The recombinant MacQ protein exhibited bifunctional acylase activity against various ranges of AHLs and against multiple β-lactam antibiotics, including penicillin G, ampicillin, and amoxicillin. The MacQ protein is comprised of 806 amino acid residues, including an N-terminal signal peptide, and belongs to the N-terminal nucleophile (Ntn) hydrolase superfamily. AHL-acylase is one of the enzymes capable of inactivating AHLs via hydrolysis of the amide bond of the acyl side-chain to produce homoserine lactone (HSL) and fatty acid. The MacQ structure clearly revealed a typical Ntn-hydrolase fold comprised of a four-layered α-β-β-α motif45 mainly composed of two polypeptide chains, α- and β-chains, generated by self-cleaving activity.

The crystal structures of MacQ, both ligand-free and in complex with the reaction products of decanoic acid (C10) and phenyl acetic acid (PAA), were determined at 2.6 Å, 2.2 Å, and 1.75 Å resolution, respectively. First, electron density was observed for the SP lying in the vicinity of the active-site pocket. This was quite unexpected, because the SP was not found in any previously reported structures of penicillin G/cephalosporin/AHL-acylases and is believed to fall away in the course of the autoproteolytic maturation. The SP atoms were refined with full occupancy, while the B-factor values of the SP were relatively high compared to those of α- and β-chain, indicating increased conformational heterogeneity or a lower occupancy of the SP as compared to the α- and β-chains. Second, the crystal structure analysis revealed that MacQ forms a high oligomeric quaternary structure. The two heterodimers consisting of the α- and β-chain are arranged face-to-face, resulting in the formation of an approximately 170-kDa capsule-shaped molecule (dimer of heterodimer) containing two SP chains. The unit-cell of the P1 lattice contains two capsule-shaped molecules, which are identical and can be superimposed with a root mean squared (RMS) difference of 0.47 Å for 1512 Cα atoms. First, the SP is observed in all heterodimeric units of MacQ in the same conformation, both in the presence and absence of ligands. Second, the residues from Gln19SP to Gly22SP form a type-II β-turn structure together with ordered solvent molecules, and the main-chain atoms that form a peptide linkage between the Val20SP and Gly21SP lie at the entrance of the hydrophobic pocket, where the residues can interact with the HSL/6-APA moiety of the bound substrate.

>[4x]SGGGDGSTYSAEIRRTTMGVPHIKAGNWGSAGYGFGYVQAQDNLCTMADSFLTYRGERSRHLGGSAQLVYNSTLGRPRNIDSDFFHRHVISDEAVDRTMAAQPAKLLQMVEGFAAGYNRYVREAKAGGSAHAACRSEAWVQPITARDVWRRIYAANLAGGYSNFAEAIANAQPPQAKA;>GAQEPAAFEPGRTRAPSLQVGGELGVG[4x];>[4x]SNMYGFGTAATGEGSGVLFGNPHWYWKGPDRFYQAQLTIDGEANVSGVSFLGLPVIQIGFNDSVAWSHTVSTARRFGFFQLSLVQGEPTSYLRDGVPVKMKPATITVPSRNADGSVSDVTRTLYHSEFGPLVNLAGLNPALAWSQGTAFAIRDINGENFRTLRTWMRWNQAKSLDEFIAIQKEEASIPWVNTVAVGRGSAKAWYADIGAVPNVSPAQTAACTTPFGMAVGQALPNVPFFDGSRSECDWLTDADSVQKGAVGVSRMPSLQRDDYVGNMNDSYWLANVHAPLTGYPAIFGPAGTSAQTLRTRMGHTMALERLAGTDGYAGNKATSAVVREMVLGSRVFSAERFKDEVLDLICTPAQWTVNGAAVDAAQACAVLAAWDNRGRKDSRGSHLWDEFWSRVPTASLFTVPFSAADPLNTPRGINAAAADALRQAMATAIARVGQSGYALDAPRGEVLYATRGGTRLPLYGGCGAMGYFTITCSENDITQGGYSMDGQPNASNSYMQVVSFPASGVQAHTFLTFSLSDDPASPHHGDYTKAYSAGQWLRVPFTEAEITGNADYRTATVKELEHHHHHH>[2x]GSHMRHRLFQLNREVDDLEQWIAEREVVAGSHELGQDYEHVTMLQERFREFARDTGNIGQERVDTVNHLADELINSGHSDAATIAEWKDGLNEAWADLLELIDTRTQILAASYELHKFYHDAKEIFGRIQDKHKKLPEELGRDQNTVETLQRMHTTFEHDIQALGTQVRQLQEDAARLQAAYAGDKADDIQKRENEV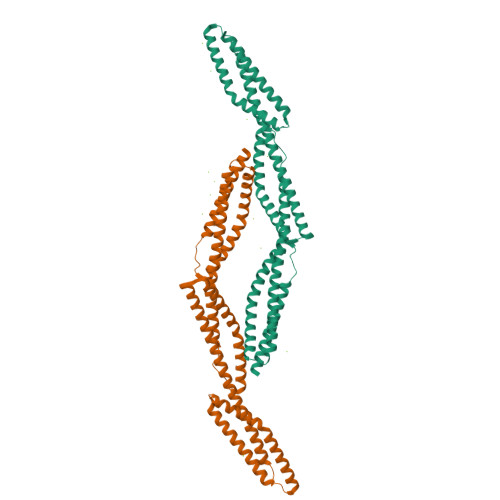LEAWKSLLDACESRRVRLVDTGDKFRFFSMVRDLMLWMEDVIRQIEAQEKPRDVSSVELLMNNHQGIKAEIDARNDSFTTCIELGKSLLARKHYASEEIKEKLLQLTEKRKEMIDKWEDRWEWLRL> TSTKRFTCPEESEASNCSCEEFPSKTHFYCPDFNPTLYVDVEDRMRVDFKCYDEPHDFKSLPNLAIGSVKLLTVVDCVLDDDRPILESFKFLEVADVRSFVYNNHENGIRYNAKYFEGMEQLENLTLARGVVSIDRDTFSGFLNLKRLTIEHNKLNLQPGTFEALSNLTYLGLVYNGLNEIQPGLFDGLESLEALSLSYNDIKSLSAGSFNGLSSLRMLNLRVNKIESFDANTFASLKELSRLEITLNPFVSLPRGLFSENKKLKTLILTNNRKLVTLPEELLANLKELTVVNLSHNGVGNLPESLLSGSSGIIELNLGYNRLNSLPEELLSDQPQLQVLNLDHNQLESIPDYFLERNVELQTLYLSHNRLRSLSEKAFTKLKNLKELHLENNQLQTIPQFLFSGTPKLEEIYMQNNQLALHANSFINEELSIADNDNTPFQVLQKLRILHLRNNSISTIFQDWYINNLEMQSLDLSFNKLPGLSYTQLQFQSNITLNLSNNEISQVLLIDDLDLQPYQRINVDLNHNPLNCNCNALKFIQLIQSKAEHGLQFNVDQLRCSEPPNLLDATMDQLQTKDLLCDFE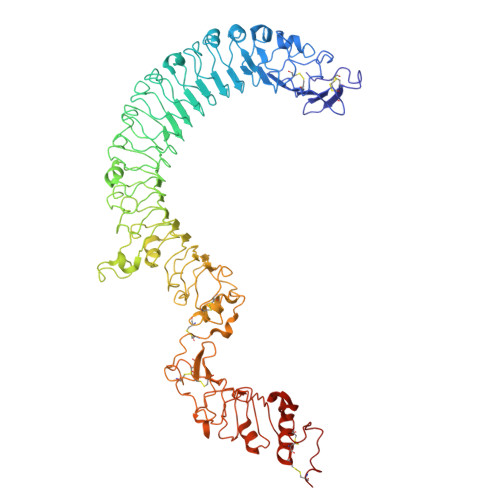SADDCPKDCQCAMRLLDHTVIVNCSGRGLTEFPDLPIPSQLHEDFNALEVHVENNRLTKLPNLTKHNEITQLYARNNSIQNLLPHNIPSKLRIIDLSQNLLKMIDDSTLAQINRSSHLETIRLSQNQWLCDCPASSFLIFVQQNSRLISDMSAIRCHPSGKSLDSITVNELCFEDYTTENLYFQ> MRGSHHHHHHGIPVSKIFFEQGTYQCLENCGTVALTIIRRGGDLTN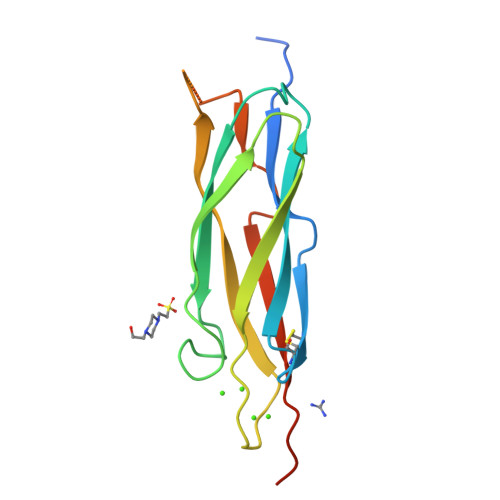TVFVDFRTEDGTANAGSDYEFTEGTVVFKPGETQKEIRVGIIDDDIFEEDENFLVHLSNVKVSSEASEDGILEANHVSALACLGSPSTATVTIFDDDHAGIFTFEE>MGVFTFEDEITSTVPPAKLYNAMKDADSITPKIIDDVKSVEIVEGNGGPGTIKKLTIVEDGETKFILHKVESIDEANYAYNYSVVGGVALPPTAEKITFETKLVEGPNGGSIGKLTLKYHTKGDAKPDEEELKKGKAKGEGLFRA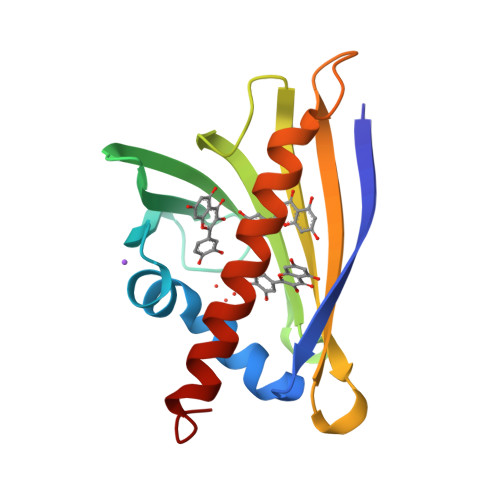IEGYVLANPTQY[3x]>GEIQWMRPSKEVGYPIINAPSKTKLEPSAFHYVFEGVKEPAVLTKNDPRLKTDFEEAIFSKYVGNKITEVDEYMKEAVDHYAGQLMSLDINTEQMCLEDAMYGTDGLEALDLSTSAGY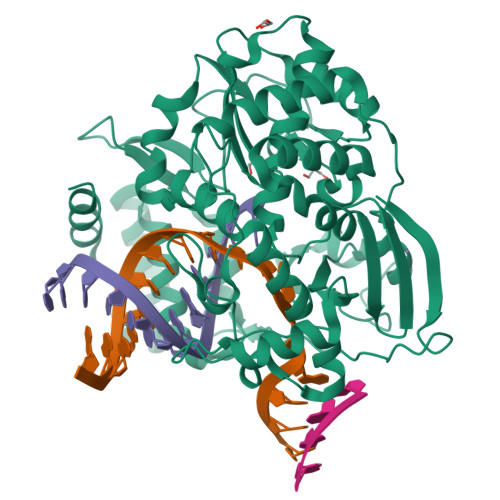PYVAMGKKKRDILNKQTRDTKEMQKLLDTYGINLPLVTYVKDELRSKTKVEQGKSRLIEASSLNDSVAMRMAFGNLYAAFHKNPGVITGSAVGCDPDLFWSKIPVLMEEKLFAFDYTGYDASLSPAWFEALKMVLEKIGFGDRVDYIDYLNHSHHLYKNKTYCVKGGMPSGCSGTSIFNSMINNLIIRTLLLKTYKGIDLDHLKMIAYGDDVIASYPHEVDASLLAQSGKDYGLTMTPADKSATFETVTWENVTFLKRFFRADEKYPFLIHPVMPMKEIHESIRWTKDPRNTQDHVRSLCLLAWHNGEEEYNKFLAKIRSVPIGRALDLPEYSTLYRRWLDSFGSSSHHHHHH[2x]> GGAMDPEFAWEKQQRKTFTAWCNSHLRKAGTQIENIDE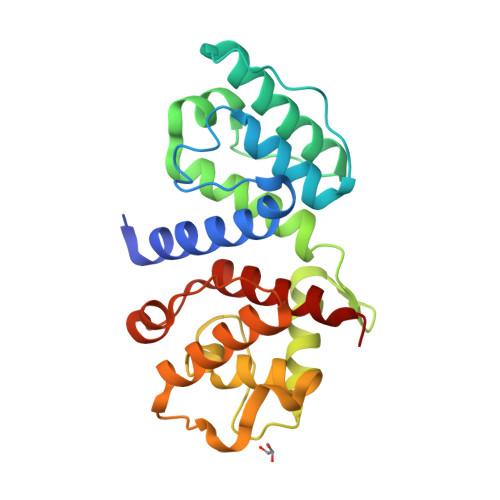DFRDGLKLMLLLEVISGERLPKPERGKMRVHKINNVNKALDFIASKGVKLVSIGAEEIVDGNAKMTLGMIWTIILRFAIQDIDVEETSAKEGLLLWCQRKTAPYKNVNVQNFHISWKDGLAFNALIHRHRPELIEYDKLRKDDPVTNLNNAFEVAEKYLDIPKMLDAEDIVNTARPDEKAIMTYVSSFYHAFSGAL> SPQPLEQIKLSESQLSGRVGMIEMDLASGRTLTAWRADERFPMMSTFKVVLCGAVLARVDAGDEQLERKIHYRQQDLVDYSPVSEKHLADGMTVGELCAAAITMSDNSAANLLLATVGGPAGLTAFLRQIGDNVTRLDRWETELNEALPGDARDTTTPASMAATLRKLLTSQRLSARSQRQLLQWMVDDRVAGPLIRSVLPAGWFIADKTGAGERGARGIVALLGPNNKAERIVVIYLRDTPASMAERNQQIAGIGAALIEHWQR

Bacterial β-lactamase enzymes are a major contributor to antibiotic resistance by hydrolyzing β-lactam antibiotics. Avibactam, which is used in combination with the β-lactam antibiotic ceftazidime, possesses a relatively broad-spectrum inhibition activity as it can inhibit class A, C, and some class D β-lactamases including extended-spectrum β-lactamases such as SHV variants. Furthermore, avibactam inhibits serine β-lactamases via a reversible mechanism which differentiates it from the currently available inhibitors. We found avibactam covalently bonded to S70 in the active site of KPC-2 and SHV-1.

In addition, we have also determined the structure of avibactam bound to SHV-1. This latter enzyme is also found in K. pneumoniae, which is often responsible for hospital-acquired infections with SHV variants demonstrating an ESBL phenotype. The structure of avibactam complexed to SHV-1 shows that this DBO inhibitor is covalently bound in a similar fashion in the active site compared to KPC-2 although there as some differences. An important difference is the sulfate moiety of avibactam makes an arginine-mediated salt bridge interaction in SHV-1 involving R244, while in KPC-2 this is absent. An additional contributing difference is that T237 in KPC-2 is more bulky than the corresponding A237 in SHV-1 and likely forces a shift in the avibactam sulfate moiety. In addition to the difference in the sulfate binding region, another variation is that Y105 in SHV-1 is disordered and occupies two conformations whereas its corresponding residue in KPC-2, W105, occupies a single conformation. In contrast, in SHV-1 and KPC-2, the avibactam N6 atom is not pointing towards its C7 atom as the distance between these atoms is greater than 3.8 Å in both structures. Also, the N6 atom of avibactam is situated further from the hydroxyl atom of S130 (i.e. 3.3 Å in SHV-1 and 3.7 Å when bound to KPC-2). In the SHV-1:avibactam complex, residue S130 is not making a strong hydrogen with avibactam, this amino acid is located at a distance of greater than 3.3 Å from the sulfate moiety. In addition to KPC-2, a similar study regarding avibactam resistance substitutions was carried out with SHV-1 β-lactamase. This latter study showed that the S130G and K234R both conferred increased resistance to avibactam/ampicillin in SHV-1.> MHHHHHHSSGRENLYFQGTYNISVVGLSGTEKEKGQCGIGKSCLCNRFVRPSADEFHLDHTSVLSTSDFGGRVVN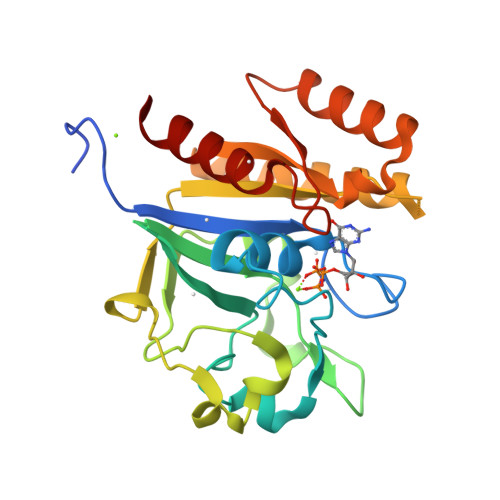NDHFLYWGEVSRSLEDCVECKMHIVEQTEFIDDQTFQPHRSTALQPYIKRAAATKLASAEKLMYFCTDQLGLEQDFEQKQMPDGKLLVDGFLLGIDVSRGMNRNFDDQLKFVSNLYNQLAKTKKPIVVVLTKCDEGVERYIRDAHTFALSKKNLQVVETSARSNVNVDLAFSTLVQLIDK>GMAADILVVDDEVDIRDLVAGILSDEGHETRTAFDADSALAAINDRAPRLVFLDIWLQGSRLDGLALLDEIKKQHPELPVVMISGHGNIETAVSAIRRGAYDFIEKPFKADRLILVAERALETSKLKREVSDLRKRTGD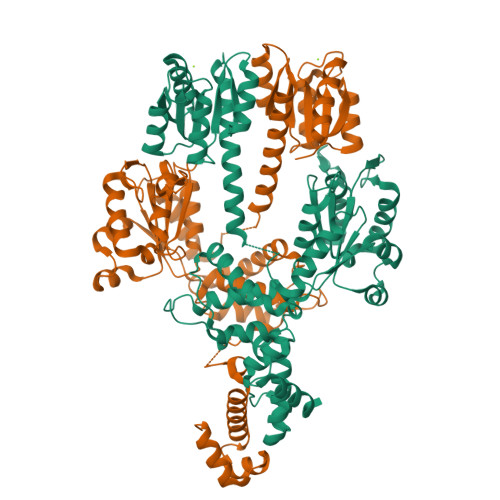QLELVGTSLAMNQLRQTIERVAPTNSRIMITGPSGAGKELVARAIHAQSSRANGPFVTVNAATITPERMEIELFGTEMDGGERKVGALEEAHGGILYLDEVADMPRETQNKILRVLVDQQFERVGGTKRVKVDVRIISSTAQNLEGMIAEGTFREDLFHRLSVVPVQVPALAARREDIPSLVEFFMKQIAEQAGIKPRKIGPDAMAVLQAHSWPGNLRQLRNNVERLMILTRGDDPDELVTADLLPAEIGDTLPRAPTESDQHIMALPLREARERFEKEYLIAQINRFGGNISRTAEFVGMERSALHRKLKSLGV[2x]> GDKLIRQ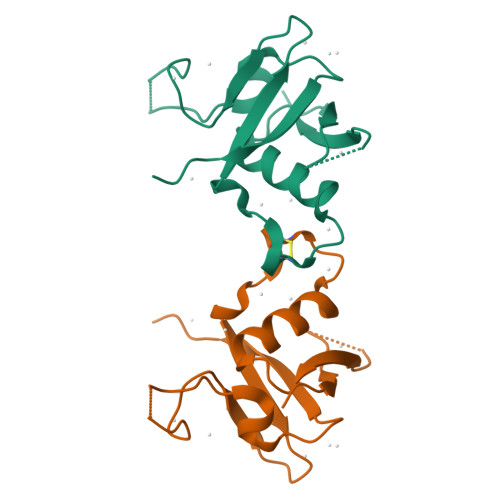QIDYKTLVLSCVSPDNANSPEVPVKILNCDTITQVKEKILDAIFKNVPCSHRPKAADMDLEWRQGSGARMILQDEDITTKIENDWKRLNTLAHYQVPDGSVVALVSKQVT> SAGINYVQNYNGNLGDFTYDESAGTFSMYWEDGVSSDFVVGLGWTTGSSNAITYSAEYSASGSSSYLAVYGWVNYPQAEYYIVEDYGDYNPCSSATSLGTVYSDGSTYQVCTDTRTNEPSITGTSTFTQYFSVRESTRTSGTVTVANHFNFWAQHGFGNSDFNYQVMAVEAWSGAGSA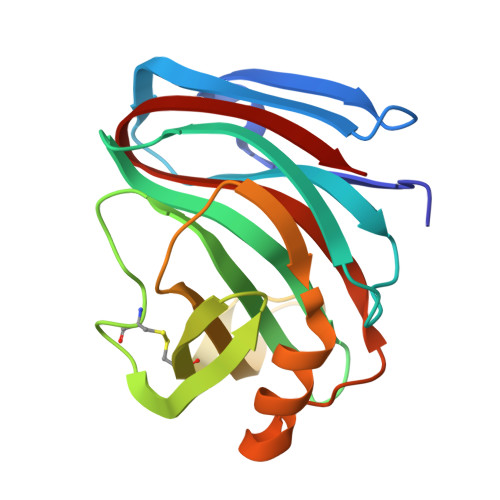SVTISS>LVSTIESRTSGDGADNFDVVSCNKNCTSGQNECPEGCFCGLLGQNKKGHCYKIIGNLSGEPPVVRR[2x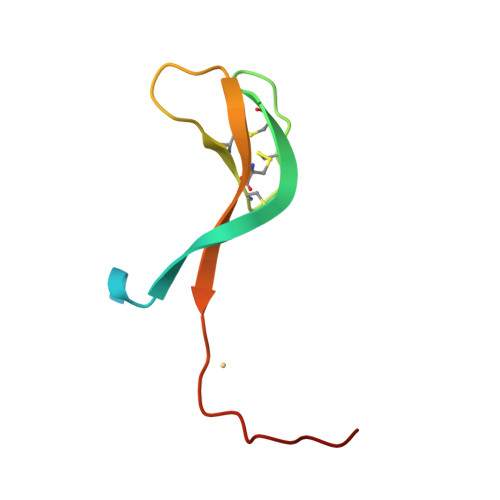]N-(2-methylpyridin-4-yl)-3-{4-[(phenylcarbamoyl)amino]-1H-pyrazol-1-yl}benzamide 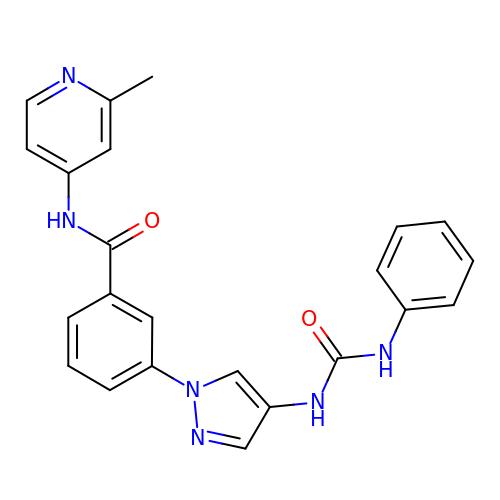| C23 H20 N6 O2 | UVLFZOYBIPADQR-UHFFFAOYSA-N>GPLGSPEFPGRPAFEGLVQRIRLIVPSTLRGGDGEAGPYSPSSLPSRCAFQFHGHDGSDESFPIEYVLRLMNDWAEVPCNPYLRIQNTGVSVLFQGFFHRPHNAPGGAITPERTNVILGSTETTGLSLGDLDTIKGRLGLDARPMMASMWISCFVRMPRVQLAFRFMGPEDAGRTRRILCRAA[2x];>GPGSQELCLHERQRYRGLFAALAQTPSEEIAIVRSLSVPLVKTTPVSLPFCLDQTVADNCLTLSGMGYYLGIGGCCPACNAGDGRFAATSR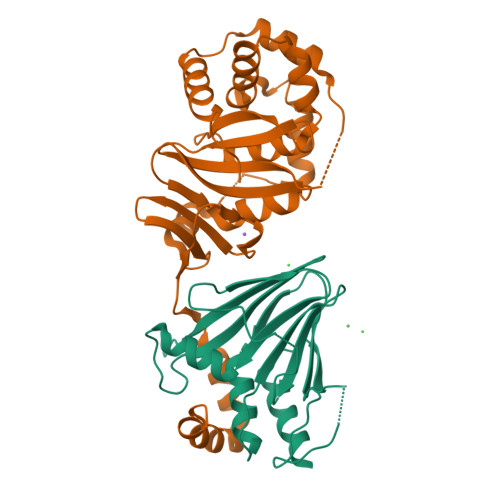EALILAFVQQINTIFEHRAFLASLVVLADRHNAPLQDLLAGILGQPELFFVHTILRGGGACDPRLLFYPDPTYGGHMLYVIFPGTSAHLHYRLIDRMLTACPGYRFVAHVWQSTFVLVVRRNAEKPTDAEIPTVSAADIYCKMRDISFDGGLMLEYQRLYATFDEFPPP[2x]> GSHMSDNEIVAGIMRDHIINLLKEGKRIDDRGFEDYRPIEIEVGVIEKAEGSALVKLGSTQVLVGIKTSLGEPFPDTPNMGVMTT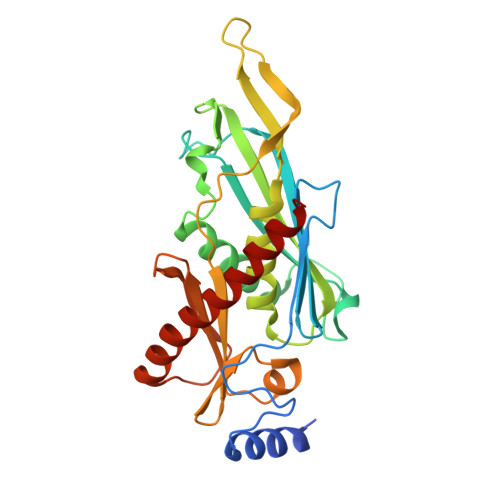NVELVPLASPTFEPGPPDERAIELARVIDRGIRESKALNLEKMVIVPGKIVRVVFIDVHVLDHDGNLMDAIGIAAIAALLNARVPKVRYNEETGEVETLDETEPLPVEKIPVPVTFAKIGNILVVDPSLDEELVMDGKITITTDETGHISAVQKSEGGAFKLEEVMYAVETAFKKAEEIRKLILEAVEKAKQ2-methylimidazo[1,2-a]pyridin-3-amine 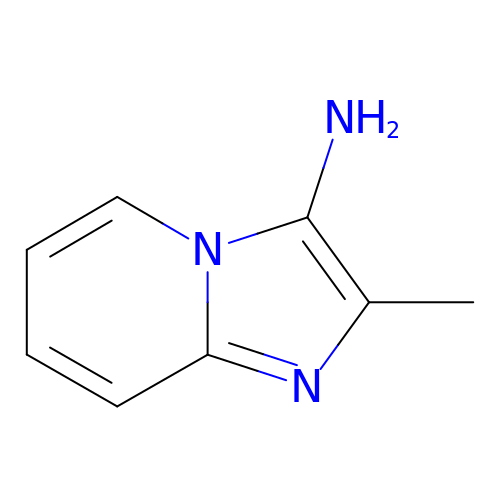| C8 H9 N3 | KTIGGQXUSNNTRK-UHFFFAOYSA-N>[2x]MGSMATLKAQHLAKSYKGRQVVRDVSMSIDSGQIVGLLGPNGAGKTTCFYMIVGLVQADQGVVRIDEQNVTHLPMHGRARAGIGYLPQEASIFRKLSVSDNIMAILETRSDLDRNGRKEALEGLLQEFHIHHIRDNLGMSLSGGERRRVEIARALASAPKFI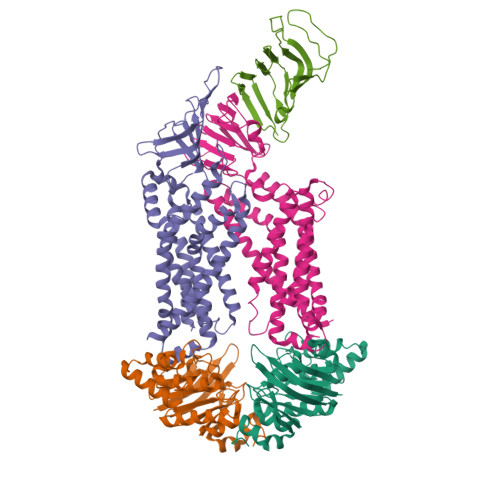LLDEPFAGVDPISVGDIKQIIHHLKAKGIGILITDHNVRETLDICETAYIVNDGQLIAEGDAESILANDLVKEVYLGHEFRLKLHHHHHH;> MGSMPKTLRQKLLLALIALLLIVAGYYWNVGLELFNEQPTRPGQDNTIDYYAENAHSLQYQEDGSLDYEMTAVKLEHQKATDITFVTTPDLLLFRGNVQPWHIQSARAEVGPKGKEVELIDDVRVARTDAKGQPSILTTTRLTVFPDKNYAQTEQAVKIDAANGVTTAVGMKAYLKDSRMHLLSNVRGQHEVR;> MGSMIVFRYLSREVLVTMSAVSAVLLVIIMSGRFIKYLAQAAQGLLDPGSLFLIMAFRIPGFLQLILPLGLFLGILLAYGRLYLESEMTVLSATGMSQKRLLGYTMAPALLVAILVAWLSLFLAPQGINQFALLLNKQDTLTEFDTLVPGRFQAMRDGTRVTYTEELSKDRGELAGIFISQKDLNSSNQERGISILVAEKGTQNIQADGSRYLILHNGYRYDGNPGQANYRAIQYDTYGVMLPKPEASSEVSERDAVPTADLFGSDNPRYQAELQWRLSTPLLVFVVTLLAVPLSRVNPRQGRFLKLLPAILLYMGYLALLIAVRGQLDKGKIPMAIGLWWVHGLFLAIGLLLFYWEPLRLKLASSRAGREVAHG;> MGSMVKLDRYIGVTVFVAILAVLGVILGLALLFAFIDELNDISASYGIGDALRFIFLTAPRRAYDMLPMAALIGCLVGLGTLASNSELTIMRAAGVSLSRIVWAVMKPMLVLMLAGILVGEYVAPWTENIAQSGRALAQGGGDSQSSKRGLWHRQGREYIHINAVQPNGVLYGVTRYRFDEQRGLESASFAKRARFETDHWQLEEVTTTLLHPREKRSEVVKLPTERWDAQLSPQLLNTVVMEPEALSISGLWQYIHYLADQGLNNNRYWLAFWTKVLQPLVTAALVLMAISFIFGPLRSVTLGQRIFTGVLVGFVFRIAQDLLGPSSLVFDFPPLLAVVIPASICALAGVWLLRRAG> MSLFNVFNVTGSAMSAESVRLNTTSSNLANADSVSSSAKDTYKARHAVFGAELSNAMRGGDTV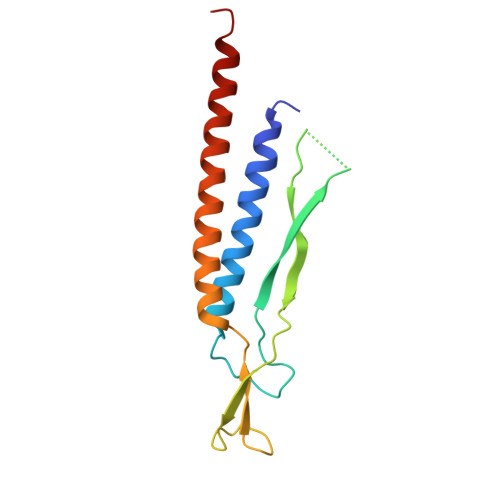PVKVMGIVESDKPLSAEYNPDHPLANEEGYIYKPNVNVMEEMANMISASRAYQTNVQVADSSKQMLLRTLQMGQ>EDNNVEGLAHLMMGDQGKS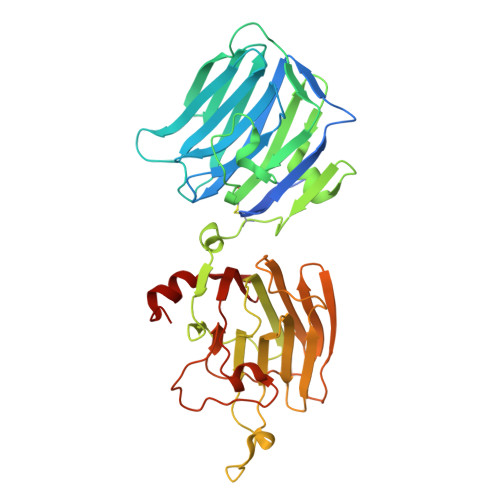KGKEEYIATFKGSEYFCYDLSQNPIQSSSDEITLSFKTLQRNGLMLHTGKSADYVNLALKNGAVSLVINLGSGAFEALVEPVNGKFNDNAWHDVKVTRNLRQVTISVDGILTTTGYTQEDYTMLGSDDFFYVGGSPSTADLPGSPVSNNFMGCLKEVVYKNNDVRLELSRLAKQGDPKMKIHGVVAFKCENVATLDPITFETPESFISLPKWNAKKTGSISFDFRTTEPNGLILFSHGKPRHQKDAKHPQMIKVDFFAIEMLDGHLYLLLDMGSGTIKIKALQKKVNDGEWYHVDFQRDGRSGTISVNTLRTPYTAPGESEILDLDDELYLGGLPENKAGLVFPTEVWTALLNYGYVGCIRDLFIDGQSKDIRQMAEVQSTAG[2x]Phosphoketolase (XPK) belongs to the transketolase family, a member of thiamine pyrophosphate (TPP)-dependent enzyme superfamily. It converts F6P, xylulose-5-phosphate (Xu5P) or sedoheptulose-7-phosphate (S7P), which are intermediates in RuBP regeneration, to produce acetyl phosphate (AcP) and C3, C4 or C5 sugar phosphates. XPK is an enzyme present in many microorganisms, primarily involved in substrate-level phosphorylation to produce AcP.

Given the importance of the physiological role of SeXPK, we solved the cryo-EM structures of SeXPK, both free (with coenzyme TPP/Mg2+ bound) and complexed with the non-hydrolyzable ATP analog, AMPPNP. In contrast to the published XPK structures from Lactococcus lactis and B. breve/longum, which exist as dimers in crystals, the cryo-EM structure of SeXPK is a dodecamer composed of six dimeric units, forming a circular donut-shaped array both for the AMPPNP-bound form and in the absence of AMPPNP. The dimer is assembled face-to-face with two AMPPNP molecules residing head-to-head at the dimer interface in-between the C terminus of the subunits, approximately 30 Å away from the catalytic site of the respective subunit (with density maps in Extended Data Fig. 5a). Comparison between the free and bound dimers in the same orientation shows that the two subunits jointly bind two AMPPNP. The key residues, H706 and Y710 from reciprocal subunits (helix α24 based on Supplementary Fig. 3), sandwich AMPPNP in the dimer interface by forming π–π stacking interactions with the adenine ring of AMPPNP. The α- and β-phosphate groups of AMPPNP are stabilized by H706, H719, R721 and R753 and the γ-phosphate group by R711 from the reciprocal subunit. Furthermore, unlike most other ATP-binding sites, there is no Asp or Glu within 5 Å of AMPPNP and no detectable divalent metal ion binding to the PPNP moiety. Instead, the negative charges of PPNP are mainly stabilized by the positive charges of the adjacent Arg and His residues. Another notable residue involved in the binding of ATP is R711, which forms a salt bridge with the γ-phosphate of ATP and explains the lack of inhibition by ADP. The root-mean-square deviation between the structures with and without AMPPNP-bound is very small: (0.42 Å from 7,897 Cα atoms of the dodecamer and 0.36 Å from 1,256 Cα atoms of the dimer). Nonetheless, ATP binding to the allosteric site could cause conformational change of active site residues through a pathway of local conformational changes involving three structurally observable steps, as summarized in Fig. 6f and detailed in Fig. 6g–n and Extended Data Fig. 5b–d, with further explanation by stereo views in Extended Data Fig. 7 showing important roles of P702–W703 in these conformational steps.

>[2x]MTSTLQATDIATLSPNEQAAIDAWWRAANYLSVGQIYLRDNPLLQEPLRPEHIKQRLLGHWGSDPGLSFVYVHLNRLIRRLDLNLIYVTGPGHGAPALLANAWLEGTYSEVYPNCQQSTAGLQQFFKQFSFPGGIGSHCTPETPGSIHEGGELGYSLSHAFGAALDNPDLIVACVIGDGEAETGPLATSWHSNKFLNPAQDGAVLPILHLNGYKIANPTLLSRISHEELRSLFIGYGYEPFFVEGNDPAILHGVMASTLATCVQKIQAIQAAARSGESSDRPMWPMIVLRTPKGWTGPATIKGHVVEGSWRSHQVPMADVLTNPEHLQLLEDWLRSYRPEELFDASGAPVAELQAIAPIGDRRMSANPVTNGGLLRRALTLPDFRDQAVSVPAPGKSRADSTRPLGQFLREVIRHNPDNFRLFGPDETASNRLDAVYEVTSKVWLGDRIPEDEDGGHLSDRGRVMEILSEHTLEGWLEAYLLTGRHGFFATYEAFAHVIDSMVNQHAKWLDVSKREVDWRAPVSSLNILLSSTVWRQDHNGFSHQDPGFIDLVTNKSARVTRIYLPPDANCLLSVADHCLRSTDYINVIVADKQSHLQYLDAEAAARHCAKGIGIWDWASNDQGASPDVVIASCGDVVTLEALAATALLREHFPDLKIRFVNVVDLFRLQPDTEHPHGLSDRDFDSLFTVDKPIIFNFHGYPWLIHKLAYRRHNHNNLHVRGYKEVGNINTPLELAIRNQVDRFNLAIDVIDRVPHLRDRGAHVKEWLKDQIHDHIQYAYQEGIDRPEINQWQWPF>[2x]MALSWNEIRRKAIEFSKRWEDASDENSQAKPFLIDFFEVFGITNKRVATFEHAVKKFAKAHKEQSRGFVDLFWPGILLIEMKSRGKDLDKAYDQALDYFSGIAERDLPRYVLVCDFQRFRLTDLITKESVEFLLKDLYQNVRSFGFIAGYQTQVIKPQDPINIKAAERMGKLHDTLKLVGYEGHALELYLVRLLFCLFAEDTTIFEKSLFQEYIETKTLEDGSDLAHHINTLFYVLNTPEQKRLKNLDEHLAAFPYINGKLFEEPLPPAQFDKAMREALLDLCSLDWSRISPAIFGSLFQSIMDAKKRRNLGAHYTSEANILKLIKPLFLDELWVEFEKVKNNKNKLLAFHKKLRGLTFFDPACGCGNFLVITYRELRLLEIEVLRGLHRGGQQVLDIEHLIQINVDQFFGIEIEEFPAQIAQVALWLTDHQMNMKISDEFGNYFARIPLKSTPHILNANALQIDWNDVLEAKKCCFILGNPPFVGKSKQTPGQKADLLSVFGNLKSASDLDLVAAWYPKAAHYIQTNANIRCAFVSTNSITQGEQVSLLWPLLLSLGIKINFAHRTFSWTNEASGVAAVHCVIIGFGLKDSDEKIIYEYESINGEPLAIKAKNINPYLRDGVDVIACKRQQPISKLPSMRYGNKPTDDGNFLFTDEEKNQFITNEPSSEKYFRRFVGGDEFINNTSRWCLWLDGADISEIRAMPLVLARIKKVQEFRLKSSAKPTRQSASTPMKFFYISQPDTDYLLIPETSSENRQFIPIGFVDRNVISSNATYHIPSAEPLIFGLLSSTMHNCWMRNVGGRLESRYRYSASLVYNTFPWIQPNEKQSKAIEEAAFAILKARSNYPNESLAGLYDPKTMPSELLKAHQKLDKAVDSVYGFKGPNTEIARIAFLFETYQKMTSLLPPEKEIKKSKGKN

MmeI is a large enzyme (919 amino acids, 105.1 kDa) that integrates DNA recognition and methyltransferase and endonuclease activities within the same polypeptide. MmeI recognizes the asymmetric DNA sequence 5’-TCCRAC-3’ (R = purine; A or G) and methylates the invariant adenine in the “top” strand (underlined). When multiple unmodified sites are encountered, MmeI cleaves the DNA approximately two helical turns downstream, on average 20 nucleotides (nts) away from the methylated adenine on the top DNA strand and 18 nts away on the bottom DNA strand (thus, TCCRAC 20/18). The Type IIG and Type IIL families comprise bifunctional R-and-M (RM) enzymes in which the two catalytic activities share the same target recognition domain (TRD) for sequence recognition.

MmeI was co-crystallized with a 29-mer DNA duplex containing a single MmeI recognition site (TCCGAC). The co-crystals were obtained in the presence of Sinefungin and diffracted to 2.6 Å resolution with synchrotron radiation. The final refined model consists of two MmeI molecules (residues 156–906), two 13-mer DNA duplexes (sense strand nucleotides 1–13 and antisense strand nucleotides 17–29), two Sinefungin molecules, two calcium ions, and a total of 61 solvent molecules. An N-terminal PD-(D/E)XK-type endonuclease domain (residues 1–155) connects to a γ-class N6-adenine DNA-methyltransferase domain (6mA-MTase; residues 301–620) via a multi-helical spacer (residues 156–300). These are followed by the TCCRAC-specific TRD (residues 621–825), and a final C-terminal helical bundle (residues 826–919). The endonuclease domain is disordered in the present structure, but its putative position—preceding the spacer—is in keeping with the ability of the enzyme to cleave DNA outside of the recognition sequence. The DNA is embedded between the TRD and the MTase domain with the adenine to be methylated (TCCGAC) flipped out of the DNA helix into the catalytic pocket of the MTase domain. The TRD makes contacts to the DNA bases primarily in the major groove, while the MTase domain makes several contacts to the DNA in the minor groove. The overall conformation of the DNA is B-DNA, but it is severely distorted at the juncture where the target adenine is flipped from the helix. To avoid catalysis and methyl transfer in our complexes, we crystallized MmeI in the presence of the AdoMet analog, Sinefungin, which has a nontransferable amino group in place of the methyl group.> MVFLPLKWSLATMSFLLSSLLALLTVSTPSWCQSTEASPKRSDGTPFPWNKIRLPEYVIPVHYDLLIHANLTTLTFWGTTKVEI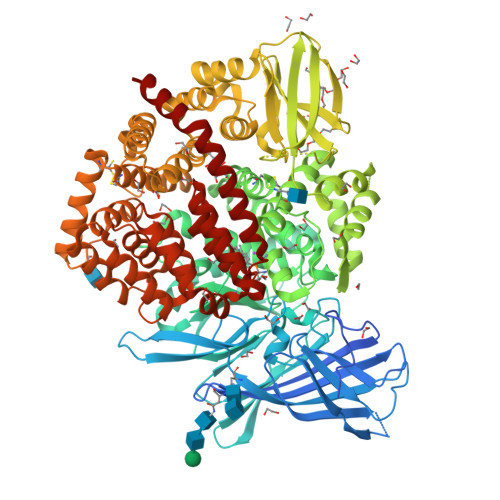TASQPTSTIILHSHHLQISRATLRKGAGERLSEEPLQVLEHPRQEQIALLAPEPLLVGLPYTVVIHYAGNLSETFHGFYKSTYRTKEGELRILASTQFEPTAARMAFPCFDEPAFKASFSIKIRREPRHLAISNMPLVKSVTVAEGLIEDHFDVTVKMSTYLVAFIISDFESVSKITKSGVKVSVYAVPDKINQADYALDAAVTLLEFYEDYFSIPYPLPKQDLAAIPDFQSGAMENWGLTTYRESALLFDAEKSSASSKLGITMTVAHELAHQWFGNLVTMEWWNDLWLNEGFAKFMEFVSVSVTHPELKVGDYFFGKCFDAMEVDALNSSHPVSTPVENPAQIREMFDDVSYDKGACILNMLREYLSADAFKSGIVQYLQKHSYKNTKNEDLWDSMASIGSGGVDVKTMMNTWTLQKGFPLITITVRGRNVHMKQEHYMKGSDGAPDTGYLWHVPLTFITSKSDMVHRFLLKTKTDVLILPEEVEWIKFNVGMNGYYIVHYEDDGWDSLTGLLKGTHTAVSSNDRASLINNAFQLVSIGKLSIEKALDLSLYLKHETEIMPVFQGLNELIPMYKLMEKRDMNEVETQFKAFLIRLLRDLIDKQTWTDEGSVSERMLRSQLLLLACVHNYQPCVQRAEGYFRKWKESNGNLSLPVDVTLAVFAVGAQSTEGWDFLYSKYQFSLSSTEKSQIEFALCRTQNKEKLQWLLDESFKGDKIKTQEFPQILTLIGRNPVGYPLAWQFLRKNWNKLVQKFELGSSSIAHMVMGTTNQFSTRTRLEEVKGFFSSLKENGSQLRCVQQTIETIEENIGWMDKNFDKIRVWLQSEK N',N'-{[(2R)-3-aminopropane-1,2-diyl]bis(oxymethanediylbenzene-3,1-diyl)}dithiophene-2-carboximidamide | C27 H29 N5 O2 S2 | 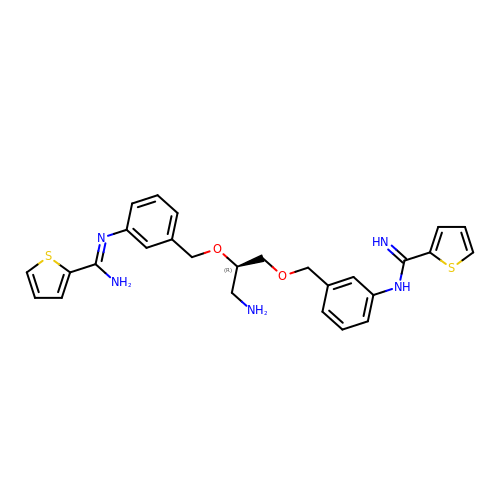KEUPBLDQGUHFOB-HSZRJFAPSA-N pyrimidin-2-ol | C4 H4 N2 O | 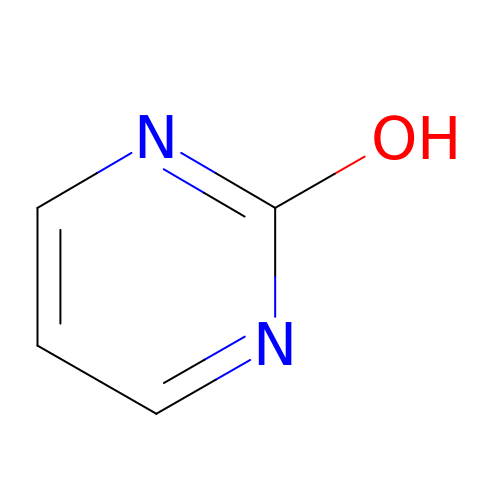VTGOHKSTWXHQJK-UHFFFAOYSA-N>MGSSHHHHHHSSGRENLYFQGHVEEKRLSAKKGLPPGTLVYTGKYREDFEIEVMNYSIEEFREFKTTDVESVLPFRDSSTPTWINITGIHRTDVVQRVGEFFGIHPLVLERILNVHQRPKVEFFENYVFIVLKMFTYDKNLHELESEQVSLILTKNCVLMFQEKIGDVFDPVRERIRYNRGIIRKKRADYLLYSLIDALVDDYFVLLEKIDDEIDVLEEEVLERPEKETVQRTHQLKRNLVELRKTIWPLREVLSSLYRDVPPLIEKETVPYFRRVYDHTIQIADTVETFRDIVSGLLDVYLSSVSNKTNEVMKVLTIIATIFMPLTFIAGIY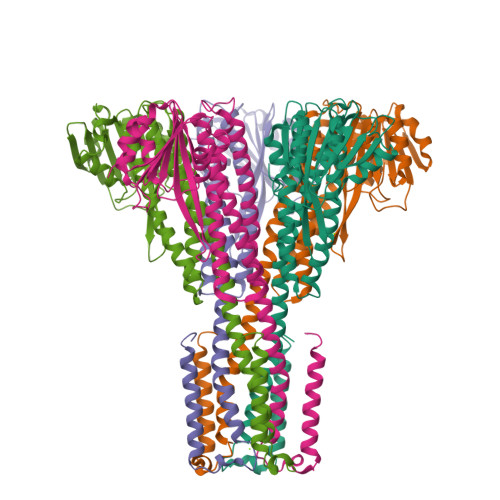GMNFEYMPELRWKWGYPVVLAVMGVIAVIMVVYFKKKKWL[5x]> QVQSVEVMRDSYGVPHVFADSHYGLYYGYGYAVAQDRLFQMDMARRSFVGTTAAVLGPGEQDAYVKYDMQVRQNFTPASIQRQIAALSKDERDIFRGYADGYNAYLEQVRRRPELLPKEYVDFDFQPEPLTDFDVVMIWVGSMANRFSDTNLEVTALAMRQSLEKQHGPERGRALFDELLWINDTTAPTTVPAPAA;> SNLWSTRPERVQEGSTVLINGPQFGWYNPAYTYGIGLHGAGFDVVGNTPFAYPIVLFGTNSEIAWGATAGPQDVVDIYQEKLNPSRADQYW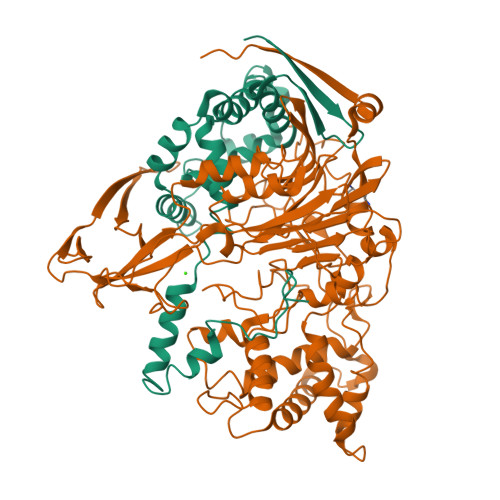FNNAWRTMEQRKERIQVRGQADREMTIWRTVHGPVMQFDYDQGAAYSKKRSWDGYEVQSLLAWLNVAKARNWTEFLDQASKMAISINWYYADKHGNIGYVSPAFLPQRPADQDIRVPAKGDGSMEWLGIKSFDAIPKAYNPPQGYLVNWNNKPAPDKTNTDTYYWTYGDRMNELVSQYQQKDLFSVQEIWEFNQKASYSDVNWRYFRPHLEKLAQQLPADDSSKAALTMLLAWDGMEQDQGGQNAGPARVLFKTWLEEMYKQVLMPVVPESHRAMYSQTGFATQQGPNPGSINLSMGTKVLLRALVLEAHPDPKRVNVFGERSSQEIMHTALQNAQARLSQEQGAQMARWTMPTSVHRFSDKNFTGTPQTMPGNTFAFTGYQNRGTENNRVVFDAKGVEFCDAMPPGQSGFTDRNGVRSPHYEDQLKLYENFECKTMDVTHADIRRNAQSSTMLLIQPQP> TINVTGDGNVFKPSAETSSTAVPSLSLSPGMLNPGGVPWIAIGDETSVTSPGALRRMTSKDIDEPLVVVTEHAIANFTKAEMALEFNREFLDKLRVLSVSPKYSDLLTYVDCYVGVS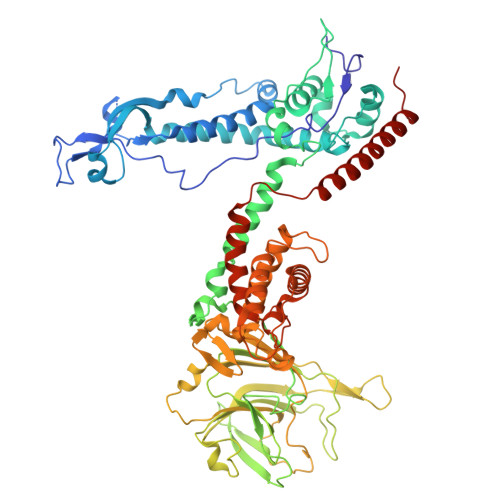ARQALNNFQKQVPVITPTRQTMYVDSIQAALKALEKWEIDLRVAQTLLPTNVPIGEVSCPMQSVVKLLDDQLPDDSLIRRYPKEAAVALAKRNGGIQWMDVSEGTVMNEAVNAVAASALAPSASAPPLEEKSKLTEQAMDLVTAAEPEIIASLVPVPAPVFAIPPKPADYNVRTLKIDEATWLRMIPKTMGTLFQIQVTDNTGTNWHFNLRGGTRVVNLDQIAPMRFVLDLGGKSYKETSWDPNGKKVGFIVFQSKIPFELWTAASQIGQATVVNYVQLYAEDSSFTAQSIIATTSLAYNYEPEQLNKTDPEMNYYLLATFIDSAAITPTNMTQPDVWDALLTMSPLSAGEVTVKGAVVSEVVPAELIGSYTPESLNASLPNDAARCMIDRASKIAEAIKIDDDAGPDEYSPNSVPIQGQLAISQLETGYGVRIFNPKGILSKIASRAMQAFIGDPSTIITQAAPVLSDKNNWIALAQGVKTSLRTKSLSAGVKTAVSKLSSSESIQNWTQGFLDKVSTHFPAP> GVDNAEKGKVSDDNASTDFVAEPVKLPENQTRVSFFYDRSTLSSVLQSTSDVSSKFTPSTAKNLQNSILLTPLPSDIVNNSVLPEQERWISFASPTTQKPPYKTKQDWNFIMFSPFTYYKCDLEVTLSKNDRETISSVVRYVPCGAPSDLSDQTMPQTPSLADTRDPHMWVVGQGTTNQISFVIPYTSPLSVLPSVWFNGFSNFDNSSRFGVAPNADFGRLLLQGQGTFSVHYRYKKMRVFCPRPTVFIPWP;> SPFPVTVREHAGTFFSTTPDTTVPVYGNTISTPFDYMCGEFTDLLSLCKIPTFLGNLDSNKKRIPYFSATNSTPATPLVTYQVTLSCSCMANSMLAAVARNFNQYRGSLNYLFVFTGSAMTKGKFLISYTPPGAGEPKTLDQAMQATYAIWDLGLNSSYNFTVPFISPTHYRQTSYNTPTITSVDGWLTVWQLTPLTYPLGVPNDSHILTLVSGGDDFTLRMPVTFTKYVPQ;> SDRVSSDTAGNTATNTQSTVGRLFGFGQRHKGKHPASCADTATDKVLAAERYYTIKLASWTKTQESFDHIRVPLPHALAGENGGVFSSTLRRHYLCKCGWRIQVQCNASQFHAGSLLVFMAPEFDTSNHSTEVEPRADTAFKVDANWQKHAQILTGHAYVNTTTKVNVPLALNHQNFWQWTTYPHQILNLRTNTTCDLEVPYVNVCPTSSWTQHANWTLVIAVLTPLQYSQGSATTIEITASIQPVKPVFNGLRHTVV;> GNEGVIINNYYSNQYQNSIDLSAN

Human Saffold virus 3 (SAFV-3) belongs to the species Theilovirus in the genus Cardiovirus of the family Picornaviridae. SAFVs cause diseases ranging from gastrointestinal disorders to meningitis. Cardioviruses have nonenveloped virions with an external diameter of about 30 nm. The major capsid proteins VP1 to VP3 form the capsid shell with pseudo-T=3 icosahedral symmetry whereas VP4 subunits are attached to the inner surface of the capsid.

The crystal structure of the SAFV-3 virion was determined to a resolution of 2.5 Å. Each of the major capsid proteins, VP1, VP2, and VP3, has a β-sandwich fold that consists of eight β-strands, conventionally named B-I, forming the two antiparallel β-sheets containing strands BIDG and CHEF. The VP4 protein of SAFV-3 contains 72 residues; however, only residues 15 to 38 could be built. The surface of the SAFV-3 virion is characterized by the presence of star-shaped plateaus around icosahedral 5-fold axes and depressions located around icosahedral 2-fold axes. In place of a continuous canyon, as seen in enteroviruses, there are five pits around each 5-fold axis in SAFV-3. The CD loop of VP1 fills the volume that corresponds to the canyon in enteroviruses. The EF loop of VP2 (residues 132 to 195), which is by convention named “puff,” is subdivided into two loops, puff A and B, in the SAFV-3 virion. Puff B contains a short α helix that has not been observed in other cardioviruses. The most prominent feature on the capsid surface formed by VP3 is a finger-like protrusion conventionally named a “knob,” which in SAFV-3 contains two β-strands. SAFV-3 contains a disulfide bond connecting cys87 and cys89 in the CD loop of VP3.> MRGSHHHHHHGSMKPYVLKFQEIRPHSEALVGGKGMNLGACSNIEGVHVPAGFC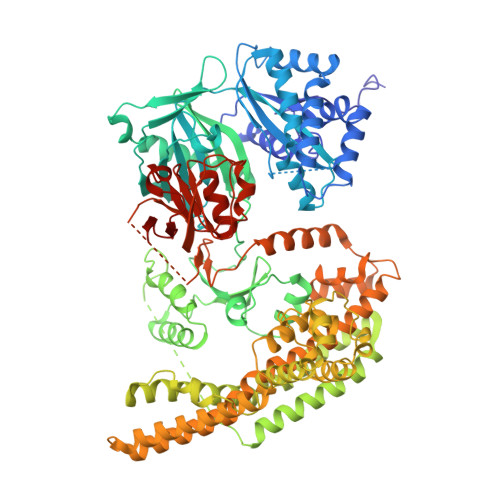LTTEAYKRTLAENNEFTQLLQRLSSLKTSDMDAIREISETIRTLIQHTQIPSEIASYMDATLLDVGGYEMPFAVRSSATAEDLPHASFAGQHDTYLNIIGKDALLQHISMCWASLFTERAIIYRIQNQFDHRKVQLAVVIQQMISPEASGILFTADPITSNRKSLSIDASFGLGEALVSGLVSADSYTVRENTITNKIIATKKLAIYSLKEGGTETRILEKSQQTKQTLTDQQIIQLAKLGRKIEAYFGKPQDIEWCLAEGAFYIVQSRPITTLYPIPEVNEPGNRVYISVAHQQMMTDAMKPLGLSFYLMTTPATMYTAGGRLFVDITQSLSAKVSRDMMVNSLGQSDPLIKDALLTVINKKGFLPPLPTEENPSHATVSGKPPVRSIPDSSSVFELVRNSENSIKHLKQSIETKSGSDLFDFIVEDLEELKRVLFNPTSIDAIMAGMDASAWLNEHIYQWLGEKNVADKLSESAPNNITSQMYLELLDVADVIRPYPAVRAYLEQTKNPDFMNELATLEGGAETKKALEDYLQKYGMRCAGEIDLTKTRWIENPLTLIPLILSNIKNFDSSASMHKFAQGEKEAFHKEQEILRRLQELPDGEQKAMETKEKIDILRHFIGYREYPKYGMINRYFIYKLALLRAGEQLVKDGILQEHEDIYFLYFEELREVVRTGQVDYELINARKRDFATFEKLTPPRILTSDGEMINGEYKRENLPKDAILGLPVSSGTVEGRARVILEMEKADLEDGDILVTAYTDPSWTPAFVSIKGLVTEVGGLMTHGAVIAREYGLPAVVGVENATTIIKDGQQIRINGTEGYIEILD> MAEKTYSGFVAIVGKPNVGKSTLLNNLLGVKVAPISPRPQTTRKRLRGILTEGRRQIVFVDTPGLHKPMDALGEFMDQEVYEALADVNAVVWVVDLRHPPTPEDELVARALKPLVGKVPILLVGNKLDAAKYPEEAMKAYHELLPEA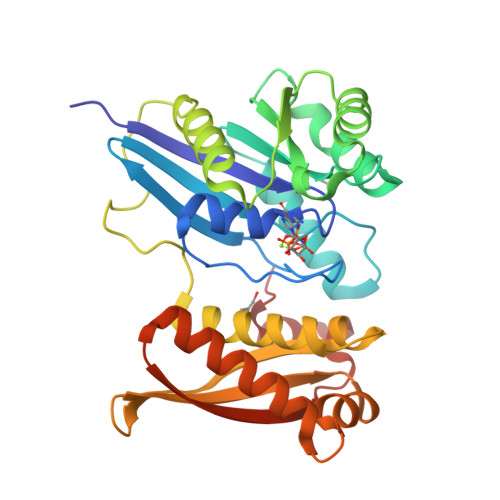EPRMLSALDERQVAELKADLLALMPEGPFFYPEDYAKSDQTFGEWVAEILREEAMKRLWHEVPYAVATKVEEVAERENGVLYIKAILYVERPSQKAIVIGEGGRKIKEIGQATRKQLEALLGKKVYLDLEVKVYPDWRKDPEALRELGYRSSVG2-{(S)-(2-chlorophenyl)[(4,4-difluorocyclohexyl)methoxy]methyl}-1H-pyrrolo[3,2-b]pyridine-7-carboxylic 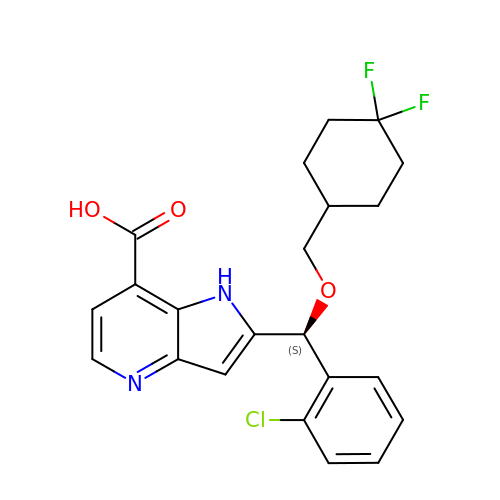acid | C22 H21 Cl F2 N2 O3 | OZTBUBVWGCXOMR-FQEVSTJZSA-N>LIEGSERLSGLTDVDEVIKDLSRLLRKLVKTRWIAVYFFDRERRDFAPARSTGLPASFLPVFREMPLAPDKIPLLKSMLRKRQHL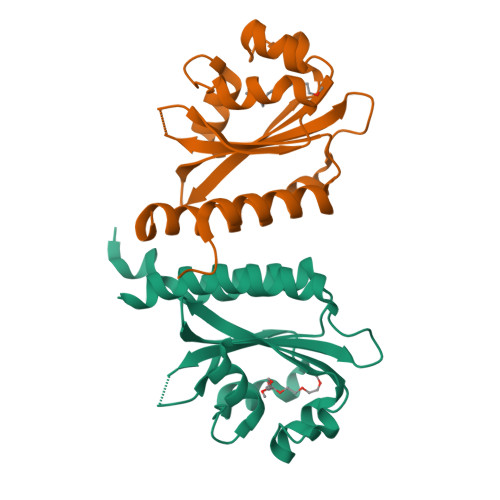MLTDPGSSDLLTPKLRKLLRNLCVLAVPMVVRTQVIGAVFMARTRDNPPFSDAETAIIRDLVSHAALVVSHMQLFDE[2x]PROTOPORPHYRIN IX 2,4-DISULFONIC ACID 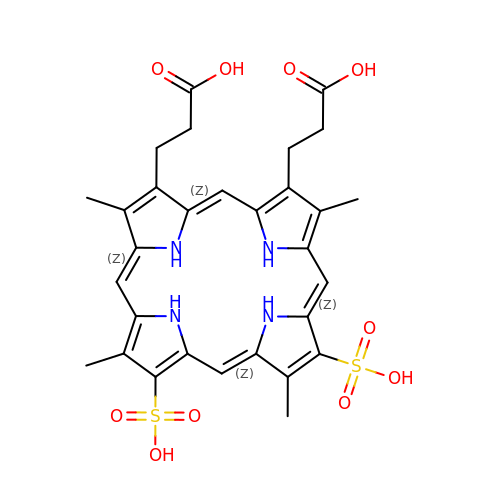| C30 H32 N4 O10 S2 | VFNOXNYLBHFZNR-IZAUZZAISA-N> NLYFQGVAIKLSSIDQFEQVIEENKYVFVLKHSETCPISANAYDQFNKFLYERDMDGYYLIVQQERDLSDYIAKKTNVKH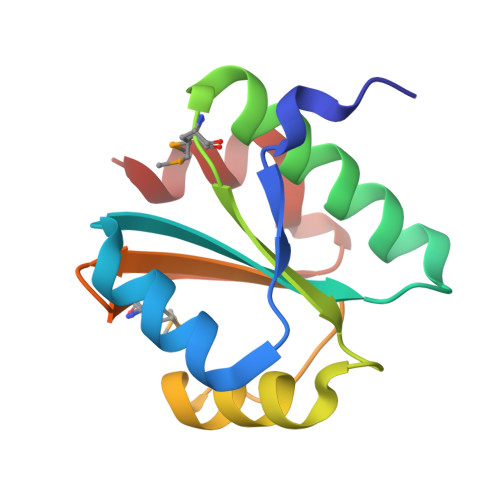ESPQAFYFVNGEMVWNRDHGDINVSSLAQAEE> PRERPHTSGHHGAGEARATAPSTVSPYGPEARAELSSRLTTLRNTLAPATNDPRYLQACGGEKLNRFRDIQCRRQTAVRADLNANYIQVGNTRTIACQYPLQSQLESHFRMLAENRTPVLAVLASSSEIANQRFGMPDYFRQSGTYGSITVE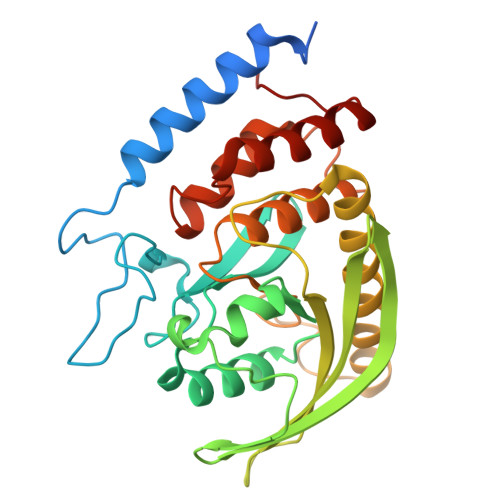SKMTQQVGLGDGIMADMYTLTIREAGQKTISVPVVHVGNWPDQTAVSSEVTKALASLVDQTAETKRNMYESKGSSAVADDSKLRPVIHCRAGVGRTAQLIGAMCMNDSRNSQLSVEDMVSQMRVQRNGIMVQKDEQLDVLIKLAEGQGRPLLNS The HIV-1 Trans-Activation Response element (TAR) RNA, located at both ends of its RNA genome, is one of the most conserved RNA structural elements in retroviruses. It assumes multiple, dynamic conformations to carry out critical functions in several stages of the HIV-1 life cycle, including reverse transcription, proviral transcription, genome dimerization and packaging, viral translation, and immune suppression, etc. Here, we report crystal structures of the full-length HIV-1 TAR which reveal substantial conformational mobility in its three conserved bulges and in its lower stem, which coordinately maintain the structural fluidity of the entire RNA. We find that TAR RNA is a robust inhibitor of PKR, and primarily uses its lower stem to capture and sequester PKR monomers, preventing their dimerization and activation.

In TAR-II, the G16A/A17G substitutions shifted the bulge one pair down to A16, which similarly permits contiguous stacking through the entire RNA. While the unpaired A17 (or A16) residue located in the mid-section is stably bulged out, the other unpaired residue, C5, located near the termini, assumed three distinct conformations among the three structures. In TAR-II, C5 is extrahelical and solvent exposed. These observations suggest that single-nt pyrimidine bulges near open dsRNA termini can exhibit considerable mobility and conformational polymorphism. Notably, among our structures, none of the three bulges interrupted the coaxial stacking that runs along the entire helical axis, which accentuates the prominent contribution of stacking in shaping RNA structures.

> GGUCUCUCUGGUUAAGCCAGAUCUGAGCCGAAAAGCUCUCUGGCUAACUAGGGAACCA> MEEPEEPADSGQSLVPVYIYSPEYVSMCDSLAKIPKRASMVHSLIEAYALHKQMRIVKPKVASMEDMATFHTDAYLQHLQKVSQEGDDDHPDSIEYGLGYDCPATEGIFDYAAAIGGATITAAQCLIDGMCKVAINWSGGWHHAKKDEASGFCYLNDAVLGILRLRRKFERILYVDLDLHHGDGVEDAFSFTSKVMTVSLHKFSPGFFPGTGDVSDVGLGKGRYYSVNVPIQDGIQDEKYYQICESVLKEVYQAFNPKAVVLQLGADTIAGDPMCSFNMTPVGIGKCLKYILQWQLATLILGGGGFNLANTARCWTYLTGVILGKTL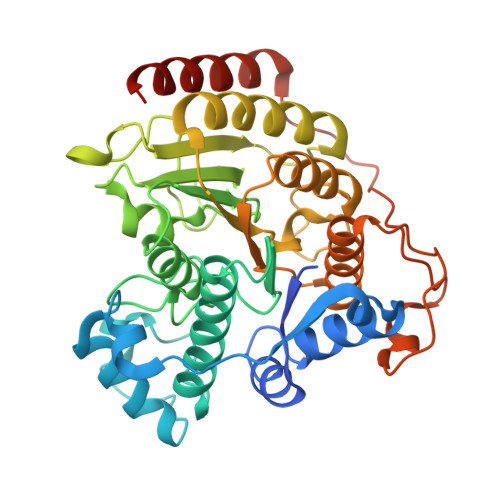SSEIPDHEFFTAYGPDYVLEITPSCRPDRNEPHRIQQILNYIKGNLKHVVIEGRGSHHHHHH>SKAVIVIPARYGSSRLPGKPLLDIVGKPMIQHVYERALQVAGVAEVWVATDDPRVEQAVQAFGGKAIMTRNDHESGTDRLVEVMHKVEADIYINLQGDEPMIRPRDVETLLQGMRDDPALPVATLCHAISAAEAAEPSTVKVVVNTRQDALYF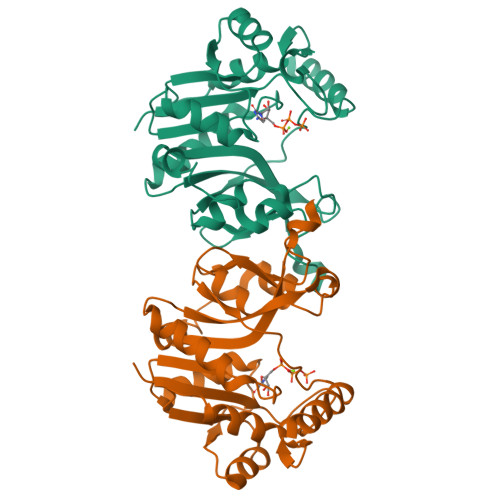SRSPIPYPRNAEKARYLKHVGIYAYRRDVLQNYSQLPESMPEQAESLEQLRLMNAGINIRTFEVAATGPGVDTPACLEKVRALMAQELAENA[2x]>[6x]M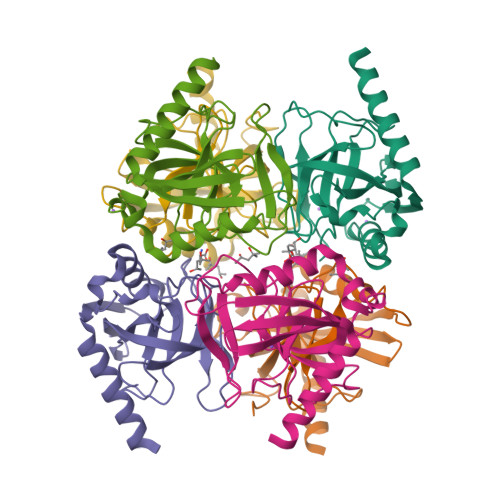AHHHHHHMSLMEIQSGRDVPNEVNVIIEIPMHGEPVKYEVDKKTGALFVDRFMTTAMFYPTNYGYIPNTLSEDGDPVDVLVITPVPLISGAVISCRAVGMLKMTDESGVDAKILAVPTTKLSKMYQSMQTYQDIPQHLLLSIEHFFKHYKDLEEGKWVKVEGWVGPDAAREEITSSINRYNHTKK> MSAISLINSGVAWFVAAAVLAFLFSFQKALSGWIAGIGGAVGSLYTAAAGFTVLTGAVGVSGALSLVSYDVQISPLNAIWLITLGLCGLFVSLYNIDWHRHAQVKCNGLQINMLMAAAVCAVIASNLGMFVVMAEIMALCAVFLTSNSKEGKLWFALGRLGTLLLAIACWLLWQRYGTLDLRLLDMRMQQLPLGSDIWLLGVIGFGLLAGIIPLHGWVPQAHANASAPAAALFSTVVMKIGLLGILTLSLLGGNAPLWWGIALLVLGMITAFVGGLYALVEHNIQRLLAYHTLENIGIILLGLGAGVTGIALEQPALIALGLVGGLYHLLNHSLFKSVLFLGAGSVWFRTGHRDIEKLGGIGKKMPVISIAMLVGLMAMAALPPLNGFAGEWVIYQSFFKLSNSGAFVARLLGPLLAVGLAITGALAVMCMAKVYGVTFLGAPRTKEAENATCAPLLMSVSVVALAICCVIGGVAAPWLLPMLSAAVPLPLEPANTTVSQP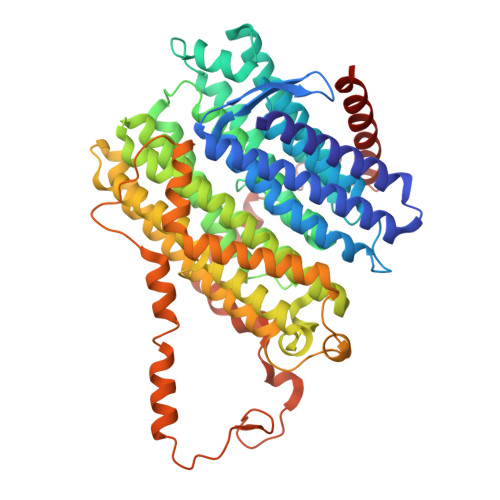MITLLLIACPLLPFIIMAICKGDRLPSRSRGAAWVCGYDHEKSMVITAHGFAMPVKQAFAPVLKLRKWLNPVSLVPGWQCEGSALLFRRMALVELAVLVVIIVSRGA> IHEGILFCIELSETMFKESSDLEYKSPLLEILESLDELMSQLVITRPGTAIGCYFYYCNREDAKEGIYELFPLRDINATFMKKLNDLLEDLSSGRISLYDYFMFQQTGSEKQVRLSVLFTFMLDTFLEEIPGQKQLSNKRVFLFTDIDKPQEAQDIDERARLRRLTIDLFDNKVNFAT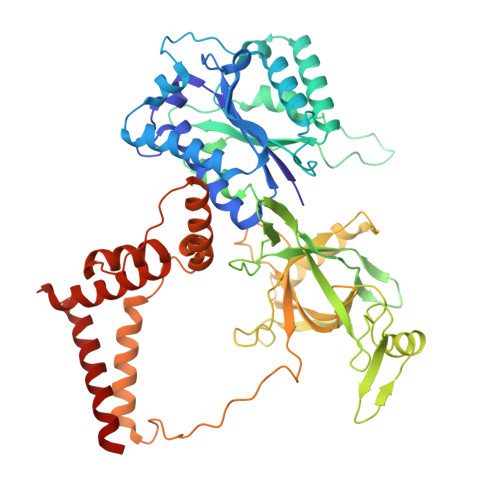FFIGYADKPFDNEFYSDILQLGSHTNENTGLDSEFDGPSTKPIDAKYIKSRILRKKEVKRIMFQCPLILDEKTNFIVGVKGYTMYTHEKAGVRYKLVYEHEDIRQEAYSKRKFLNPITGEDVTGKTVKVYPYGDLDINLSDSQDQIVMEAYTQKDAFLKIIGFRSSSKSIHYFNNIDKSSFIVPDEAKYEGSIRTLASLLKILRKKDKIAILWGKLKSNSHPSLYTLSPSSVKDYNEGFYLYRVPFLDEIRKFPSLLSYDDGSEHKLDYDNMKKVTQSIMGYFNLRDGYNPSDFKNPLLQKHYKVLHDYLLQIETTFDENETPNTKKDRMMREDDSLRKLYYIRNKILESEKSEDPIIQRLNKYVKIWNMFYKKFNDDN> GSHMSNTQTVLPFTGLNTPNGVAVDSAGTVYVTDHGNNRVVKLAAGSNTQTVLPFTGLNTPNGVAVDSAGTVYVTDHGNNRVVKLAAGSNTQTVLPFTGLNTPNGVAVDSAGTVYVTDHGNNRVVKLAAGSNTQTVLPFTGLNTPNGVAVDSAGTVYVTDHGNNRVVKLAAGSNTQTVLPFTGLNTPNGVAVDSAGTVYVTDHGNNRVVKLAAGSNTQTVL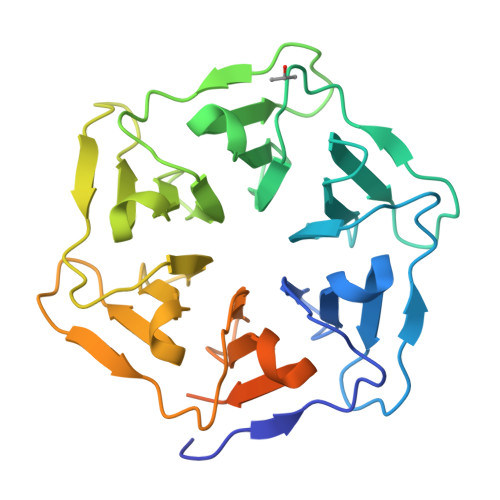PFTGLNTPNGVAVDSAGTVYVTDHGNNRVVKLAAGSNTQTVLPFTGLNTPNGVAVDSAGTVYVTDHGNNRVVKLAAG> GDPIKILMPSLSPTMEEGNIVKWLKKEGEAVSAGDALCEIETDKAVVTLDASDDGILAKIVVEEGSKNIRLGSLIGLIVEEGEDWKHVEIPKD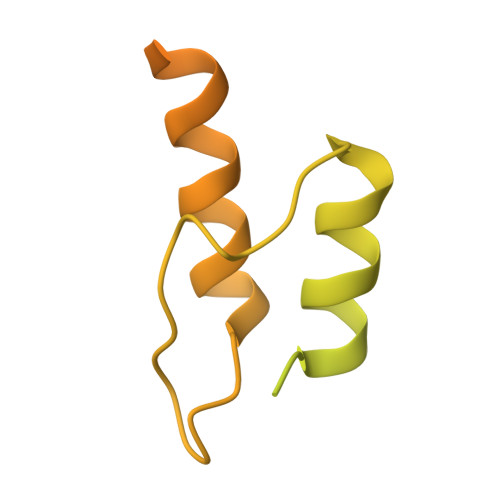VGPPPPVSKPSEPRPSPEPQISIPVKKEHIPGTLRFRLSPAARNILEKHSLDASQGTATGPRGIFTKEDALKLVQLKQTGKITESRPTPAPTATPTAPSPLQATSGPSYPRPVIPPVSTPGQPNAVGTLEHHHHHH>GSNMKAVCVMTGTAGVKGVVKFTQETDNGPVHVHAEFSGLKAGKHGFHVHEFGDTTNG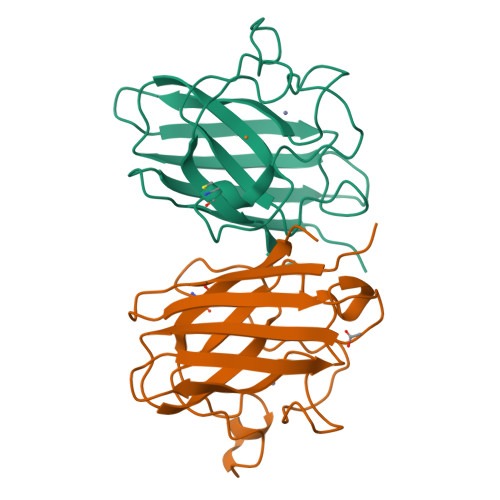CTSAGAHFNPTKQEHGAPEDSIRHVGDLGNVVAGADGNAVYNATDKLISLNGSHSIIGRSMVIHENEDDLGRGGHELSKVTGNAGGRLACGVVGLAAE[4x]> GPDKYRTRLLHLKGKKHIRVHEVPKTYKSLNSGDVFVLDAGKTVIQWNGAKAGLLEKVKAAELLQAIEGEREGIASGRVVAEADNDTEFFTLLGDKGPIADAAAGGSDLEADKKDQPAVLLRLSD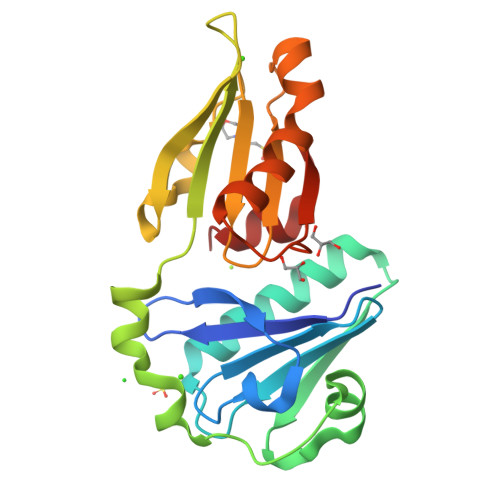ASGKFEFTEVARGLKVKRNLLDSNDVFVLYTGAEVFAWVGKHASVGEKKKALSFAQEYVQKAGLPIHTPVARILEGGENEVFEDFFD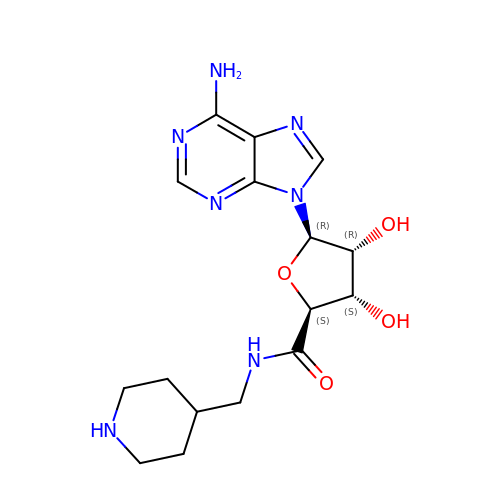(2~{S},3~{S},4~{R},5~{R})-5-(6-aminopurin-9-yl)-3,4-bis(oxidanyl)-~{N}-(piperidin-4-ylmethyl)oxolane-2-carboxamide | C16 H23 N7 O4 | QORMXDVXCHKGRB-MEQWQQMJSA-N>MEQPFDLAAELAKQPHLLEIAGNLLMKSGPEDYIGAVLCLRGTLYFKKAHTPLVRESLCQCFDEFERLAEPHLTWLWREEPAQGKPLTAYRDTQPLREMMGAMDEDDHLSFCYTSGKKSRDAGAWLFDIYGKRSWQAKMGHD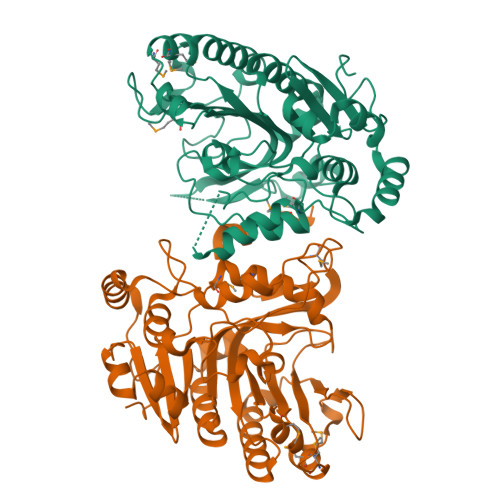LSVLEFSVPLLYQERQPLDFLQLFIDFARRLEPEQGYAGHAYNLSPTSWDNDEPSEAFMAARMPGLDVGTACLLANTPEFKPTRIKTVSWLTLLNNERLALAGGLDALRAQLPSSHFAFYRYGDGVVIQAGAYPYIAGDAEDSRPAPYVLLNHALKGIRYETIGSLHGGSHDGELRLVGWAADQWLKRLDVEDSEIPRWCDKLLSAEPYLDATNTLPERL[2x]> MEELQKSIGHKPEPTDEEWELIKTVTEAHVATNAQGSHWKQKRKFLPEDIGQAPIVNAPEGGKVDLEAFSHFTKIITPAITRVVDFAKKLPMFCELPCEDQIILLKGCCMEIMSLRAAVRYDPESETLTLNGEMAVTRGQLKNGGLGVVSDAIFDLGMSLSSFNLDDTEVALLQAVLLMSSDRPGLACVERIEKYQDSFLLAFEHYINYRKHHVTHFWPKLLMKVTDLRMIGACHASRFLHMKVECPTELFPPLFLEVFED

The human (h) TR exists in two isoforms, hTRα (NR1A1), and hTRβ (NR1A2). hTRα is expressed at higher levels in heart and plays a major role in regulation of heart rate, whereas TRβ is the predominant isoform that is expressed in the liver and pituitary and is involved with hepatic cholesterol metabolism and regulation of metabolic rate. Thyroid receptor (TR) activation occurs when an agonist ligand such as TH or similar compounds binds to a hydrophobic pocket in the core of its ligand-binding domain (LBD). This causes conformational changes which allow DNA bound receptors to interact with coactivators, mediating transcription.

In hTRβ, Arg282 from helix 3, and Arg316 and Arg320 from helix 6 interact with the GC-1 oxyacetic acid carboxylate both directly and via water-mediated hydrogen bond interactions, as previously observed in a previous hTRβ/GC-1 structure. Asn331 forms a hydrogen bond with Arg282 that anchors the latter in place and permits it to form a stable interaction with the GC-1 carboxylate group. In TRβ a single productive conformation is observed, in which the ligand interacts strongly with Arg282, while this residue interacts with the carbonyl group of Asn331. For hTRβ the residue oscillates around a mean defined value, indicating a single conformation. The second strongest interaction is the hydrogen bond that Arg282 forms with the Asn331 residue in the hTRβ isoform (-19 kcal/mol). In hTRβ, Arg282 interacts, at the same time, with the carboxylate of the ligand and with the side chain of Asn331, which locks in place the productive conformation of the former residue. Therefore, the stabilization of the productive conformation resulting from the Arg282-Asn331 interaction is of key importance for hTRβ selectivity of GC-1. On the other hand, the productive conformation of Arg282 with GC-1 in hTRβ is very stable both in X-ray structure and in MD simulations, being locked in place by the strong interaction of the side-chain of Asn331.>MEYHVAKTGSDEGKGTLKDPFLTINKAASVAMAGDTIIVHEGVYREWVKPKYKGLSDKRRITYKAAEGEKVVIKGSERIQSWQRVEGNVWRCQLPNSFFGEFNPYKEEVFGDWLLTVNEKKHLGDVYLNGMSFYEVTNYEDLFNPQLRTEVLDHWTQKIVPIKNAEQTKYVWYAEVDREKTTIYANFQGADPNEEFVEINVRRSCFYPVETGIDYITVKGFEMAHAATPWAPPTADQPGLIGPNWSKGWIIEDNIIHDAKCSAISIGKEATTGNNYRSIRKDKPGYQYQLEAVFNAKRNGWSKEKIGSHIIRNNTIYDCGQNAIVGHLGGVFSEIYNNHIYNIALKREFYGHEIAGIKLHAAIDVQIHHNRIHDCSLGLWLDWEAQGTRVSKNLFYNNNRDVFVEVSHGPYLVDHNILSSEYAIDNMSQGGAYINNLIAGKMNQRKVLNRSTQYHLPHSTEVAGFAFVYGGDDRFYNNIFIGKEGLENVGTSHYNNCTTSLEEYIEKVNEVPGDLGEFERVEQPVYINKNAYFNGAEPFEKEKDNLVKKDFDPKLAIIDEGDEVYLSLQLPDEFENI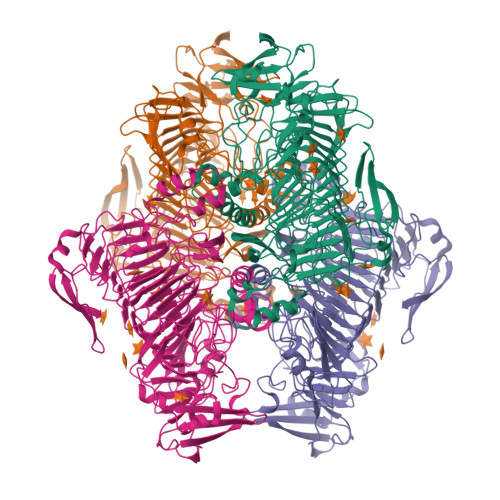VGDIHSTKTLERVRIVDAEYESPDGKELVLDTDYLDAKKPENSSIGPIALLKKGNNYIKVW[4x]>HHHHHHSSGLVPRGSHMTDIRSETAELRAELVERVHKFGPVFADGVAEGERERRLPDATVRAIDQSQLAMLWTAKSYGGLETDVRTMSEVAKVLSHYCPSTSWVVNNVNGSNLLASKFPRAALDEVFGDAPGAKLASVFAAAGTAVRTPGGYRLTGSWPYGTGILHDDWAILVAREVDADGEPVGGLSMLVPARDLTVEDTWHTVGMRATGSHTVVLRDTFVPEHRVISGELQRSRESATDLGLPPLFRTAAIAAMAVVCASVVLGAGQAARALVVEKAPTRGIAPSKYTRQTDSRTFVSSLGRTALSIDAAEMHVARAATALDDAAYDAVALPDSELLRIRGDVGQAVSLVTTALDELLWAHGAASFAESNPLQRYWRDANTAARHAMLNVHVGHELYGGSFFGLDPIVPSL[24x]

In vitro characterization, bioinformatics and structural investigations revealed that XiaF is a new member of the group D FMOs, monooxygenases that receive reduced FAD/FMN from a NAD(P)H-dependent flavin reductase and assemble in a tetrameric ACAD-fold composed of N- and C-terminal helical domains and a central β-sheet domain35. At the heart of the biosynthetic pathway, however, we discovered an unusual cyclization cascade involving the non-canonical terpenoid cyclases XiaE and XiaF22. Here we report the in vitro reconstitution of XiaF and a designated flavoenzyme-reductase, which jointly mediate a cryptic indole hydroxylation step that has been proposed to be a key step in non-canonical terpenoid cyclization. Accordingly, in the terpenoid pathway C-3 hydroxylation of the indole ring of indosespene by C4a-hydroperoxyflavin as the electrophilic oxygenating species yields a reactive intermediate (most likely the 3-hydroxyiminium cation 9, although deprotonation to yield an hydroxyindolenine intermediate is also conceivable) that is prone to nucleophilic attack of the exo-methylene group, resulting in the pentacyclic intermediate 16.

The structure of XiaF was solved at 2.4 Å resolution applying molecular replacement (Rfree=22.9%, search model: 4-hydroxyphenylacetate 3-hydroxylase, PDB ID: 2JBS48). A similar conformation of FAD has been previously reported for an FAD synthase from yeast49. This bent conformation is missing the distinct interactions between the FADH2’s β-phosphate and the amino acids Tyr144, Arg266 and Ala350. Instead, three new intramolecular H-bonds between the ribose and adenine moieties of the cofactor are formed (3.0, 2.6 and 3.0 Å). Therefore, it is unclear whether this unique bent conformation has a biological function.[(2~{R},3~{S},4~{S},5~{R})-3,4-bis(oxidanyl)-5-[3-[4-[4-(trifluoromethyloxy)phenyl]-1,2,3-triazol-1-yl]propyl]oxan-2-yl]methyl ~{N}-[(2~{S})-2-azanyl-4-methyl-pentanoyl]sulfamate 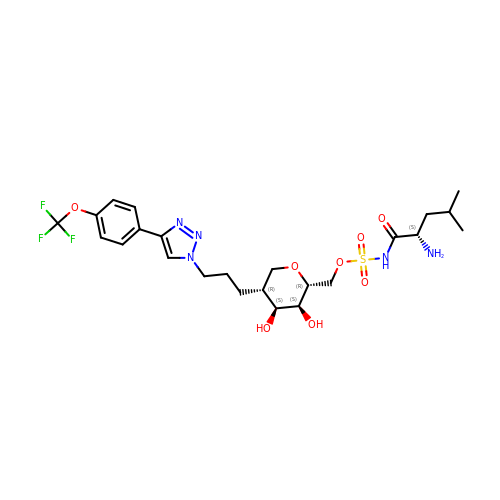| C24 H34 F3 N5 O8 S | RYNRVLDROIFGBF-RCUFNAHASA-N> FNLDAEAPAVLSGPPGSFFGFSVEFYRPGTDGVSVLVGAPKANTSQPGVLQGGAVYLCPWGASP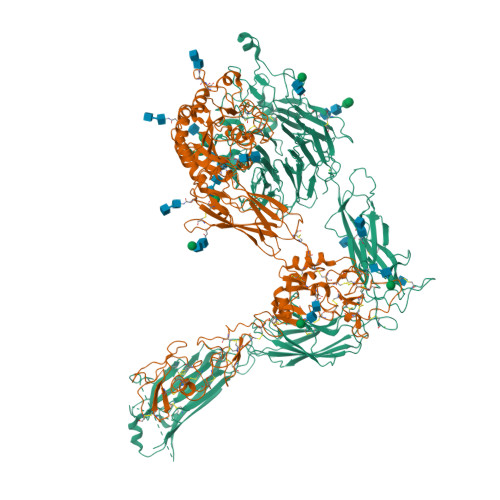TQCTPIEFDSKGSRLLESSLSSSEGEEPVEYKSLQWFGATVRAHGSSILACAPLYSWRTEKEPLSDPVGTCYLSTDNFTRILEYAPCRSDFSWAAGQGYCQGGFSAEFTKTGRVVLGGPGSYFWQGQILSATQEQIAESYYPEYLINLVQGQLQTRQASSIYDDSYLGYSVAVGEFSGDDTEDFVAGVPKGNLTYGYVTILNGSDIRSLYNFSGEQMASYFGYAVAATDVNGDGLDDLLVGAPLLMDRTPDGRPQEVGRVYVYLQHPAGIEPTPTLTLTGHDEFGRFGSSLTPLGDLDQDGYNDVAIGAPFGGETQQGVVFVFPGGPGGLGSKPSQVLQPLWAASHTPDFFGSALRGGRDLDGNGYPDLIVGSFGVDKAVVYRGRPIVSASASLTIFPAMFNPEERSCSLEGNPVACINLSFCLNASGKHVADSIGFTVELQLDWQKQKGGVRRALFLASRQATLTQTLLIQNGAREDCREMKIYLRNESEFRDKLSPIHIALNFSLDPQAPVDSHGLRPALHYQSKSRIEDKAQILLDCGEDNICVPDLQLEVFGEQNHVYLGDKNALNLTFHAQNVGEGGAYEAELRVTAPPEAEYSGLVRHPGNFSSLSCDYFAVNQSRLLVCDLGNPMKAGASLWGGLRFTVPHLRDTKKTIQFDFQILSKNLNNSQSDVVSFRLSVEAQAQVTLNGVSKPEAVLFPVSDWHPRDQPQKEEDLGPAVHHVYELINQGPSSISQGVLELSCPQALEGQQLLYVTRVTGLNCTTNHPINPKGLELDPEGSLHHQQKREAPSRSSASSGPQILKCPEAECFRLRCELGPLHQQESQSLQLHFRVWAKTFLQREHQPFSLQCEAVYKALKMPYRILPRQLPQKERQVATAVQWTKAEGSYGVPLWIIILAILFGLLLLGLLIYILYKLGFFKRSLPYGTAMEKAQLKPPATSDA;> QTDENRCLKANAKSCGECIQAGPNCGWCTNSTFLQEGMPTSARCDDLEALKKKGCPPDDIENPRGSKDIKKNKNVTNRSKGTAEKLKPEDIHQIQPQQLVLRLRSGEPQTFTLKFKRAEDYPIDLYYLMDLSYSMKDDLENVKSLGTDLMNEMRRITSDFRIGFGSFVEKTVMPYISTTPAKLRNPCTSEQNCTTPFSYKNVLSLTNKGEVFNELVGKQRISGNLDSPEGGFDAIMQVAVCGSLIGWRNVTRLLVFSTDAGFHFAGDGKLGGIVLPNDGQCHLENNMYTMSHYYDYPSIAHLVQKLSENNIQTIFAVTEEFQPVYKELKNLIPKSAVGTLSANSSNVIQLIIDAYNSLSSEVILENGKLSEGVTISYKSYCKNGVNGTGENGRKCSNISIGDEVQFEISITSNKCPKKDSDSFKIRPLGFTEEVEVILQYICECECQSEGIPESPKCHEGNGTFECGACRCNEGRVGRHCECSTDEVNSEDMDAYCRKENSSEICSNNGECVCGQCVCRKRDNTNEIYSGKFCECDNFNCDRSNGLICGGNGVCKCRVCECNPNYTGSACDCSLDTSTCEASNGQICNGRGICECGVCKCTDPKFQGQTCEMCQTCLGVCAEHKECVQCRAFNKGEKKDTCTQECSYFNITKVESRDKLPQPVQPDPVSHCKEKDVDDCWFYFTYSVNGNNEVMVHVVENPECPTGPDIIPIVAGVVAGIVLIGLALLLIWKLLMIIHDRREFAKFEKEKMNAKWDTGENPIYKSAVTTVVNPKYEGK> MEQRITLKDYAMRFGQTKTAKDLGVYQSAINKAIHAGRKIFLTINADGSVYAEEVKDGE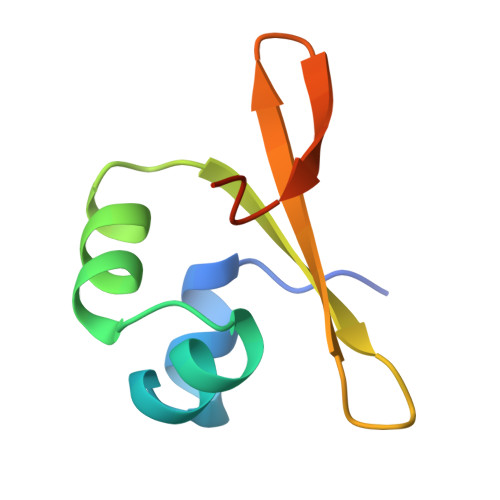VKPFPSNKKTTA> MSSAFSGLKIPELSVDPAEVFKSDNPQLVSVLLDEFELQEQRPFFSGLIPEKQINIALKKSPQLKKLACHLLEAYEINGRRWKHADRRRVLEKAIRLLEKVSNELKGDIQKLENNVKESGKDSEELNKTREKHGEILADMGRAYLHRAKII;> MGSSHHHHHHSQDPMQHIIPLTITFLESFRVIEWHKSSDRNSLRFLRGYAYARWHRSLKNNKGRPYITGTLVRSAIIRAAEELLWLNDGNYKGAICCPGEFNGSNAKVFREGKARRLRRRQTLTWPTKCACHEKEPCPFCLLLGRYEKSSKTSKSPVLNNVNFSNFNVLGKEKEFLNIEDVADMRVVNRVDQQSGKAEDFFNIWEITDGAWKIFRGEIQVSDKGWSDEENFSKFLTLLKGASVLVDKISGGLCYLTLDKPELAELPAVKTEKDVLEPGDDASVLEISRPPYWNNMLNLAGTISEAFEREDKLVHLRLFADTVRELRRSDIETLDLPKGHADRLGKPSDHFIWDIEINKKVKLRNWLFWIFNEFRDTYAYFDWRTFCEALGQALYLEAKKQVPNQFSSERPVGATPAMEVKTPEHDPGRAAQGPRYEWLIKGELVSQTPFFFGWSTEADNREHTNLKLLAARDGRLRLPLSVLRGILRRDIKVVLDNKCRAELAMKQPCSCPVCNLMKKITIRDSFSSNYAEPPKIRHKIRLDPKSGTVAKGALFDSEVGPRGVVFPFELRLRSADDTLPQALKTVFSWWQQGTVSFSGDAGTGKGIFCLRNLKSIRWDLKTEMDKYAATLGGRKTPVGKWDKCHIPDDKTYPWVKETVEISVCSPFITKDPVNSLIDSAGYDAICYTTVDLEKSENINSLPESEISLLFEMFDLQYPMSYLFPNKDIYLLKGESFRGMLRTAVGRGENLLLREHEDCSCTLCRIFGNEHNAGKIRVEDFIIQGEPRTKLVDRVAIDRFTAGAKDKFKFDAAPIVGTPTNKLKFRGNIWIHRDLDGLACESLKLALEDIENGLYPFGGLGNAGFGWVNYNPLSHPAQEENKADFSLTKKMELNWSMKELSTDKIYWPHYFLPFGKKVLREKTPPSHACIDENEDSELYSGKIVCTLETRTPLIIPDSEFQGEEHKSYDFFNLNGELCIPGSEIRGMISSVFEALTNSCMRIFDEKKRLSWRMNPNKKDKKNNNRRELDDFIPGRVTNDRKMEEMKEYRYPFYDQAITANDKQNKYFDQWEATIELTDESLEKLKAEKILQSVLDALRPLTKKKEKYKNTETFVFDLKKFIGKIDDNQQMISEALERGKVRLTGNSLKQISKTKKIPRQILNQLKGLKDNTYENREQFISVLKTTVRGINDEQISLILDNIDEDVRLTDLSLTKIRKAKVPQTLVDMLADLKKDEPYKNEKEFLSEFKKKMGEIIGLILKHAAKTGGDVPRYNHPTPTDKMLLSLAAYNRNHKHENGKAEYRIVKPKHNLKVDFMFAVTPFENPFKGYNPAAVVEEPVGGYLKVSGPNKIEKVKKVNPNSVSVRDDKNQEIIHNGVYLRKITVANAKSKNKLRERLVPEFAWYDKDSEAAYAMTKRCERVFVEIGAKPIPIQPSAREKFKILTQEYQKNAKQQKTPEAFQTILPKDGELRPGDLVYFREDKKTNTVTDIIPVRISRTVDDEVLARKIPDDVGDVRPCVREILDKEKQKEIADAGVKEVFQHHPDGLCPACSLFGTTFYKGRIAFGFAFHKDKDPELANNGKHITLPLLERPRPTWSMPKKESRVPGRKFYVHHQGWERVIKHSNLDESDPNATKQTVNNRSVQAIKEEQKFQFEVRFENLREWELGLLVYVLQLEPQFAHKLGMGKALGFGSVRIRVGEIHSGPKELDESRLVSSAMKKMEEIWDRDKNVLEKLFRLLYFNESKDIKVRYPKLQKEKEEEEEESGYMELAKEEYQPEQRRNKLTNPWEGWGNILKKPAILI

In the present study, we use cryoelectron microscopy to determine structures of the Desulfonema magnum (Dm) Craspase complex to gain mechanistic insights into its regulation. We used cryoelectron microscopy (cryo-EM) to analyze the Craspase complex, which resulted in two structures, one showing clear density for crRNA and all protein domains of the complex (DmCas7-11–crRNA and DmTPR-CHATfull), whereas the second lacks density for the regions of DmTPR-CHAT (DmCas7-11–crRNA and DmTPR-CHATNTD). DmTPR-CHAT makes multi-domain interactions with DmCas7-11–crRNA via its NTD and CTD, forming two major binding sites. The overall structure of D. magnum Craspase revealed that the complex adopts a ‘closed’ conformation characterized by the steric occlusion of the first segment of the spacer crRNA by the CLD.

Cryo-EM data processing of the Craspase complex revealed flexibility of the TPR and CTD, in contrast to the NTD which is rigidly bound to the complex. These findings show that the NTD is sufficient for the association of DmTPR-CHAT with DmCas7-11–crRNA. The NTD interacts with the Cas7.4 palm, a loop extending from the Cas7.3 palm, and the insertion finger from Cas7.4 via salt bridges and hydrogen bonds. Asp310 or Asp307 (CLD) and Lys1526 (insertion finger) form a salt bridge facilitated by interactions between the insertion finger and the NTD. This network of interactions stabilizes the CLD. Strikingly, the highly conserved amino acid Asp682 implicated in nuclease activity is proximal to this region, indicating that target cleavage occurs nearby. We also show that the inhibitory role of DmTPR-CHAT is mediated by its NTD.> MSQVSTRLVRLLNMVPYFQANPKVTRAEAAAALGVTGKQLDADLDQLWMCGLPGYSPGDLIDFDFVGDTIEVTFSAGVDHPLRLTSTEATGILVALRALVDVP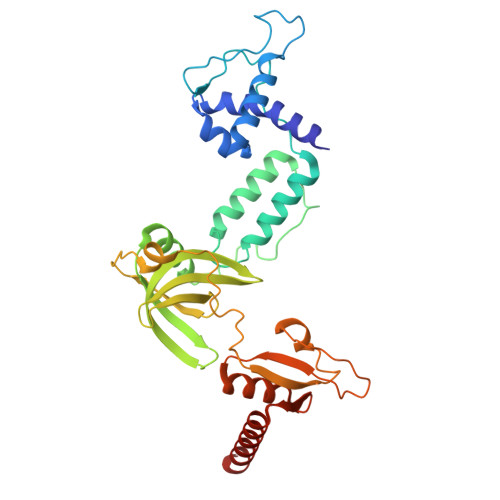GMVDPEAARSAIAKIESAVGSQRAVVEGITEDTSAEPGAAATVRTAVRENRALTLEYYSASRDSLATRTVDPIRVVLVGDNSYLEAWCRSAEAVRLFRFDRIVDAQLLDDPAAPPPPAVAAGPDTSLFDADPSLPSATLLIGAAAAWMFDYYPLRDITERPDGSCEATMTYASEDWMARFILGFGAEVQVLAPESLATRVRQAAEAALQAYARCV> GSHMASEGPALYEDPPDQKTSPSGKPATLKIASWNVDGLRAWIKKKGLDWVKEEAPDILCLQETKCSENKLPA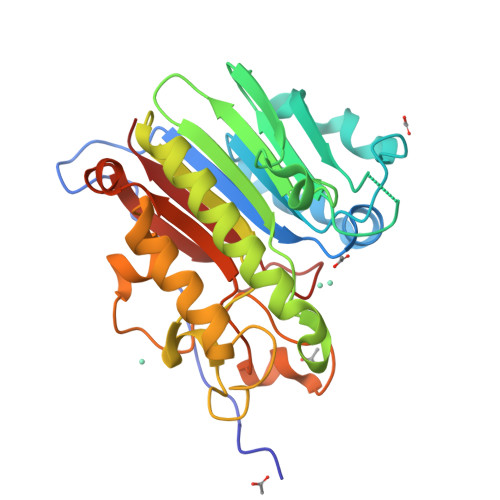ELQELPGLSHQYWSAPSDKEGYSGVGLLSRQCPLKVSYGIGDEEHDQEGRVIVAEFDSFVLVTAYVPNAGRGLVRLEYRQRWDEAFRKFLKGLASRKPLVLCGDLNVAHEEIDLRNPKGNKKNAGFTPQERQGFGELLQAVPLADSFRHLYPNTPYAYTFWTYMMNARSKNVGWRLDYFLLSHSLLPALCDSKIRSKALGSDHCPITLYLAL> NEKLAKKKIVSIDAGRKYFSPEQLKEIIDKAKHYGYTDLHLLVGNDGLRFMLDDMSITANGKTYASDDVKRAIEKGTNDYYNDPNGNHLTESQMTDLINYAKDKGIGLIPTVNSPGHMDAILNAMKELGIQNPNFSYFGKKSARTVDLDNEQAVAFTKALIDKYAAYFAKKTEIFNIGLDEYANDATDAKGWSVLQADKYYPNEGYPVKGYEKFIAYANDLARIVKSHGLKPMAFNDGIYYNSDTSFGSFDKDIIVSMWTGGWGGYDVASSKLLAEKGHQILNT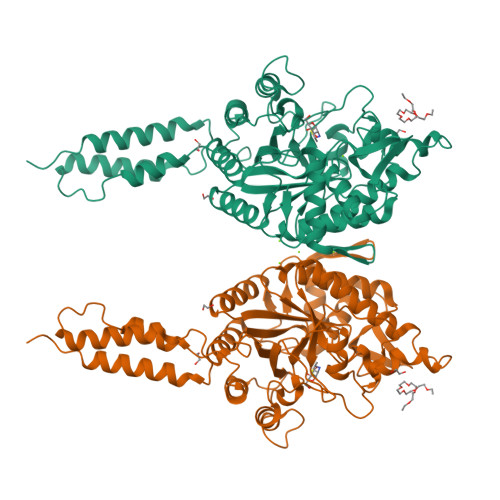NDAWYYVLGRNADGQGWYNLDQGLNGIKNTPITSVPKTEGADIPIIGGMVAAWADTPSARYSPSRLFKLMRHFANANAEYFAADYESAEQALNEVPKDLNRYTAESVTAVKEAEKAIRSLDSNLSRAQQDTIDQAIAKLQETVNNLTLTP> GIDPFTMSGDGSPPIHTRRQGFDPADELRAAGTLTKISIGSGADAETTWLAAGHAVVRQVLGDHKRFSTRRRFDRRDEIGGTGVFRPRELVGNLMDYDPPEHTRLRHLLTPGFTQRRMRRLAPRIEEIVTDRLDAMEQAGPPADLIELFADEVPGAVLCELIGVPRDDQAMFLQLCHRHLDASLSARKRAAAGEAFARYLVAMMARERKDPGDGFIGSIVAEHGDTITDEELRGVCVQLMLAGDDNVSGMIGLGVLALLRHPEQIAALRGDDQSADRAVDELIRYLTVPYAPTPRTAVEDVMVADQVIKEGETVLCSLPMANRDRALLPDADRLDVTRTPVPHVAFGHGIHHCLGAALTRLQLRIAYTALWRRFPALQLADPAQEIMFRTSTPAYGLTSLLVAW;> GAMGRPALEAVTRPERVPLTARQLRAWLLARPSEETRGRHLSVALRLRGRLDVAALEAALRDVAARHEILRTTFPGDAQTVHQHIHDAAPV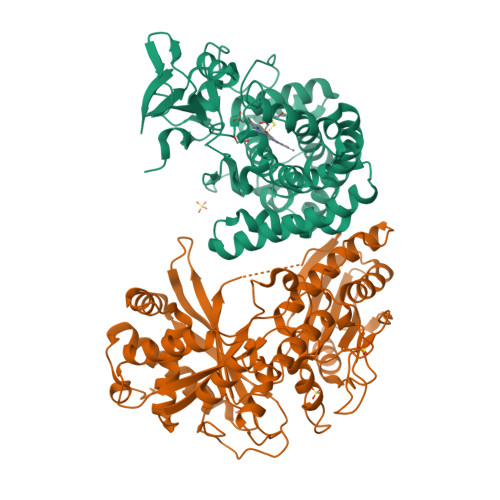RLTPVPATEEDLPARLAERGEQLFDLTRDMPWRCELFALSEKEHVLSVTVHRIAADDDSMDVFFRDLAAAYGARRAGRAPERAPLALQFADYAIWEQRLLDGEREQDSLINDQITFWRNHLAGIDQETVLPFDRARPAIPSRRAGTVALRLDAGPHARLAEAVESAGADMPQLVQAALAMLLTRYGAGTDLVIGTTLPRDEDLIDLEPMIGPFARPFPVRTDLSADPTFLEVVARVQEAVREARQHLDVPFEKIPELLALPGSLSRHPVYQVGLQVREEDNGAWDAAELPALRTSVEPTGVEAIELDLAFALTERRNDDDDEDGIEGALHYAADLFDHDTAASLARRLVRVLEQVAEDPGRRISDLDILLDDAERGAPLESAWSHPQFEK Members of the presynaptic neurexin (NRX) and postsynaptic neuroligin (NL) transmembrane protein families form the axis of a signaling pathway that is crucial for the formation and function of excitatory and inhibitory synapses throughout the brain. MDGA proteins bind NLs and control their function and interaction with NRXs via unknown mechanisms. MDGA proteins are attached to the postsynaptic membrane via a C-terminal GPI anchor, and their large (∼900 amino acids) extracellular domain consists of six immunoglobulin-like domains (Ig1-6), a fibronectin type III-like (FnIII7) domain, and a memprin, A5, mu (MAM8) domain. The extracellular region of the NLs contains a cholinesterase-like domain that forms a stable interaction with the α/β-NRX1-3 LNS6 (laminin, NRX, sex-hormone-binding globulin) domain (Araç et al., 2007, Chen et al., 2008, Fabrichny et al., 2007).

Simultaneously, the insertion point for SSB in NL1 is in close proximity to the Site I interface (Koehnke et al., 2010), suggesting that presence of SSB might affect MDGA binding. Next, we determined the crystal structure of human NL1 containing SSB (hNL1(+B)) at 2.55 Å. The nine-residue SSB (NRWSNSTKG), inserted between Gly295 and Leu305, was clearly visible in the electron density; the N-linked glycan at Asn300, a modulator of the NL-NRX interaction (Chih et al., 2006, Comoletti et al., 2003), was, however, not fully resolved due to conformational flexibility. Superposition of NL1(+B) and NL1-MDGA1 (0.308 Å RMSD over 434 NL1 Cα positions) or NL1-NRX1 (0.306 Å RMSD over 428 NL1 Cα positions) structures revealed that SSB is spatially immediately adjacent to both Site I interfaces. We found, using SPR, that insertion of SSB weakened the NL1-MDGA1-2 interaction ∼7-fold, while reducing the NL1-β-NRX1(±4) interaction less than 2-fold. We propose that this differential effect is due to the much larger molecular footprint of MDGA and the resulting close proximity of the MDGA Ig5 and Ig6 domains to the N-linked glycan at Asn300, suggesting that SSB reduces the NL-MDGA interaction due to steric hindrance. Indeed, removal of the N-linked glycan (Asn300Gln mutant) partially recovered the NL1-MDGA1-2 interaction affinity, whereas it had almost no effect on the NL1-β-NRX1(±4) interaction. Taken together, our results suggest that, despite the proximity of SSB to the Site I interface, its presence does not eliminate the ability of MDGA to block NL-NRX signaling. Rather, SSB provides a way to fine-tune the NL1-MDGA1-2 interaction at excitatory synapses.

>ETGQKLDDVDPLVATNFGKIRGIKKELNNEILGPVIQFLGVPYAAPPTGERRFQPPEPPSPWSDIRNATQFAPVCPQNIIDGRLPEVMLPVWFTNNLDVVSSYVQDQSEDCLYLNIYVPTEDDIRDSGGPKPVMVYIHGGSYMEGTGNLYDGSVLASYGNVIVITVNYRLGVLGFLSTGDQAAKGNYGLLDLIQALRWTSENIGFFGGDPLRITVFGSGAGGSCVNLLTLSHYSEGNRWSNSTKGLFQRAIAQSGTALSSWAVSFQPAKYARMLATKVGCNVSDTVELVECLQKKPYKELVDQDIQPARYHIAFGPVIDGDVIPDDPQILMEQGEFLNYDIMLGVNQGEGLKFVENIVDSDDGISASDFDFAVSNFVDNLYGYPEGKDVLRETIKFMYTDWADRHNPETRRKTLLALFTDHQWVAPAVATADLHSNFGSPTYFYAFYHHCQTDQVPAWADAAHGDEVPYVLGIPMIGPTELFPCNFSKNDVMLSAVVMTYWTNFAKTGDPNQPVPQDTKFIHTKPNRFEEVAWTRYSQKDQLYLHIGLKPRVKEHYRANKVNLWLELVPHLHNLNDRTKHHHHHH[2x]> GVLGLEAQAVPYYEKAIAS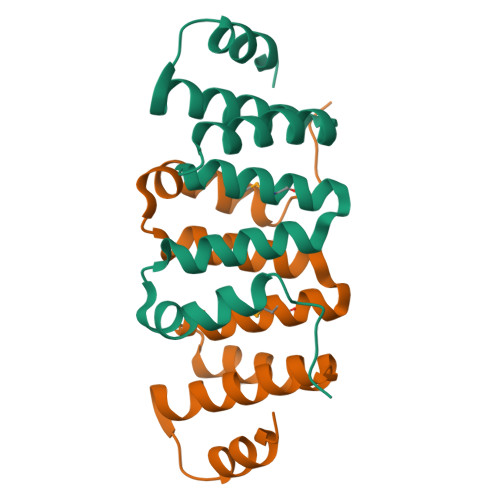GLQGKDLAECYLGLGSTFRTLGEYRKAEAVLANGVKQFPNHQALRVFYAMVLYNLGRYEQGVELLLKIIAETSDDETIQSYKQAILFYADKLDETWKA>[2x]DLRRQLRKAVM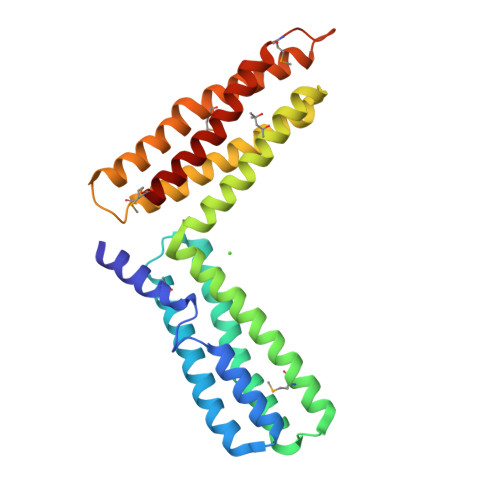DHVSDSFLETNVPLLVLIEAAKNGNEKEVKEYAQVFREHANKLIEVANLACSISNNEEGVKLVRMSASQLEALCPQVINAALALAAKPQSKLAQENMDLFKEQWEKQVRVLTDAVDDITSIDDFLAVSENHILEDVNKCVIALQEKDVDGLDRTAGAIRGRAARVIHVVTSEMDNYEPGVYTEKVLEATKLLSNTVMPRFTEQVEAAVEALSSDPAQPMDENEFIDASRLVYDGIRDIRKAVLMI> MRGSHHHHHHGSACMFSNKTRQDSIQKMQQEELDLLIIGGGITGAGVAVQAAASGIKTGLIEMQDFAEGTSSRSTKLVHGGIRYLKTFDVEVVADTVGERAVVQGIAPHIPKPDPMLLPIYEDEGATTFNMFSVKVAMDLYDKLANVTGTKYENYTLTPEEVLEREPFLKKEGLKGAGVYLDFRNNDARLVIDNIKKAAEDGAYLVSKMKAVGFLYEGDQIVGVKARDLLTDEVIEIKAKLVINTSGPWVDKVRNLNFTR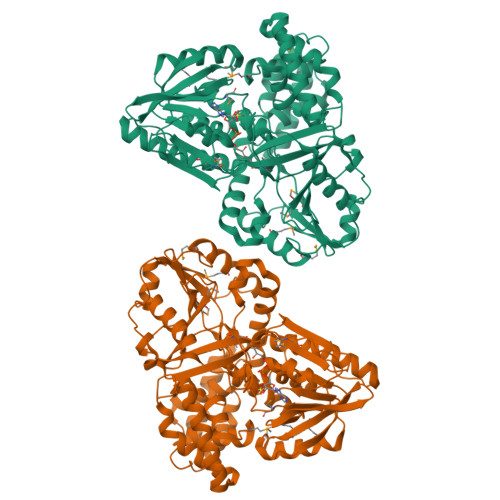PVSPKMRPTKGIHLVVDAKKLPVPQPTYFDTGKQDGRMVFAIPRENKTYFGTTDTDYQGDFTDPKVTQEDVDYLLDVINHRYPEANITLADIEASWAGLRPLLIGNSGSPSTISRGSSLEREPDGLLTLSGGKITDYRKMAEGALRLIRQLLKEEYGIETKEIDSKKYQISGGNFDPTKLEETVTELAKEGVAAGLEEEDATYIADFYGTNARRIFELAKEMAPYPGLSLAESARLRYGLEEEMVLAPGDYLIRRTNHLLFERDQLDEIKQPVIDAIAEYFGWTEEEKAQQTKRLEALIAESDLRELKGEK>[4x]GMKGISHRIAIP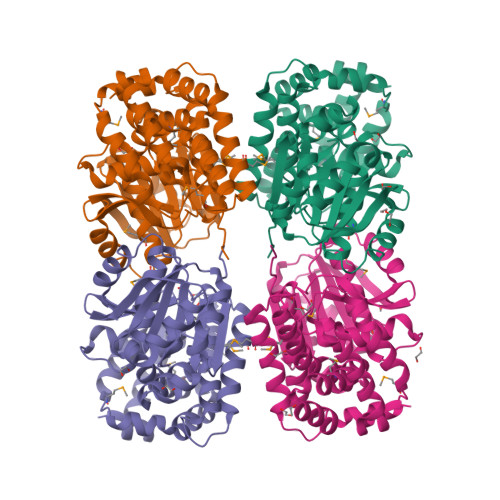LILEVGNNKIYNIGQIIKKGNFKRVSLYFGEGIYELFGETIEKSIKSSNIEIEAVETVKNIDFDEIGTNAFKIPAEVDALIGIGGGKAIDAVKYMAFLRKLPFISVPTSTSNDGFSSPVASLLINGKRTSVPAKTPDGIVVDIDVIKGSPEKFIYSGIGDLVSNITALYDWKFEEENHKSIIDDFAVMISKKSVNSFVRTDFKSIKDEVFLKELVDSLTMNGIAMEIAGNSSPASGAEHLISHALDKFLPNPQLHGIQVGVATYIMSKVHKHREERIKKILSDTGFFNYVKGLNMKKSDFKRAISEAHLIKPARYTYLHVEKNCETAKEIVDTDEILRNILV> KETAAAKFERQHMDSSTSAASSSNYCNQMMKSRNLTKDRCKPVNTFVHESLADVQAVCSQKNVACKNGQTNCYQSYSTMSITACRETGSSKYPNCAYKTTQANKHIIVACEGN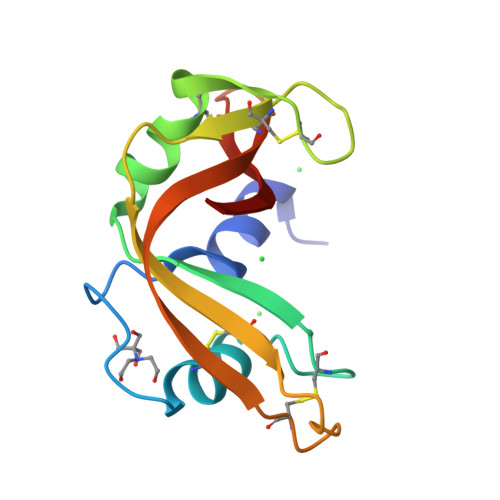PYVPVHFDASV> CRTSCPLALASYYLENGTTLSVINQNLNSSIAPYDQINFDPILRYNSNIKDKDRIQMGSRVLVPFPCECQPGDFLGHNFSYSVRQEDTYERVAISNYANLTTM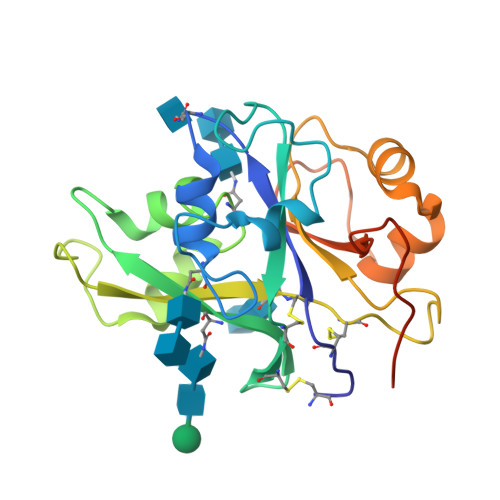ESLQARNPFPATNIPLSATLNVLVNCSCGDESVSKDFGLFVTYPLRPEDSLSSIARSSGVSADILQRYNPGVNFNSGNGIVYVPGRDPNGAFPPFKSSKQDGVHHHHHH> GPFPPPGMSLPEYWGEEHVWWDGRAAFHGEVVRPACTLAMEDAWQIIDMGETPVRDLQNGFSGPERKFSLRLRN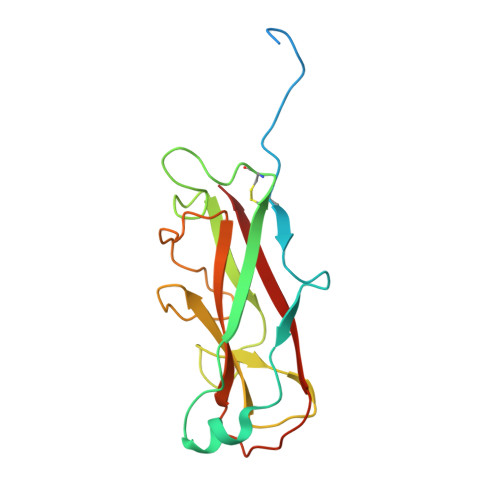CEFNSQGGNLFSDSRIRVTFDGVRGETPDKFNLSGQAKGINLQIADVRGNIARAGKVMPAIPLTGNEEALDYTLRIVRNGKKLEAGNYFAVLGFRVDYE Bile salt hydrolases (BSHs) comprise a diverse family of microbial enzymes that catalyse critical BA transformation. Primary conjugated BAs synthesized in the liver, such as the tauro- and glycoconjugates of cholic acid (TCA, GCA), are deconjugated by BSHs to generate cholic acid (CA) (BA names and abbreviations are summarized in Supplementary Fig. 1). We found that Lactobacillaceae BSHs display a clear bias for either glycine or taurine-conjugated BAs. Notably, each monomer contains a loop that swaps into the active site of a neighbouring monomer within the tetramer and places amino acids proximal to the catalytic residues.

To examine the molecular foundations of BSH substrate specificity, we determined the crystal structures of six of the Lactobacillaceae BSHs examined above: four glycine-preferring (LgasBSHb, LaciBSHa, LingBSH, LreuBSH) and two taurine-preferring (LgasBSHa, LjohBSHc) BSHs. We examined the sequences of these loops and found that taurine-preferring enzymes exclusively contained G-V/T-G (‘G-X-G’) motifs, while glycine-preferring enzymes solely contained S-R-G/S (‘S-R-X’) motifs. The glycine-preferring enzyme clade containing LaciBSHa, LcriBSHa and LcriBSHb exhibits the highest activity.

>[4x]MCTSIIFSPKDHYFGRNLDLEITFGQQVVITPRNYTFKFRKMPSLKKHYAMIGISLDMDDYPLYFDATNEKGLGMAGLNYPGNATYYEEKENKDNIASFEFIPWILGQCSTISEVKDLLSRINIADLNFSEKMQASSLHWLIADKTGTSLVVETDKDGMHIYDNPVGCLTNNPQFPKQLFNLNNYADVSPKMPKNNFSDKVNMAGYSRGLGSHNLPGGMDSESRFVRVAFNKFNAPIAETEEENIDTYFHILHSVEQQKGLDEVGPNSFEYTIYSDGTNLDKGIFYYTTYSNKQINVVDMNKEDLDSSNLITYDMLDKTKFNHQNHHHHHH>[2x]SQIPASEQET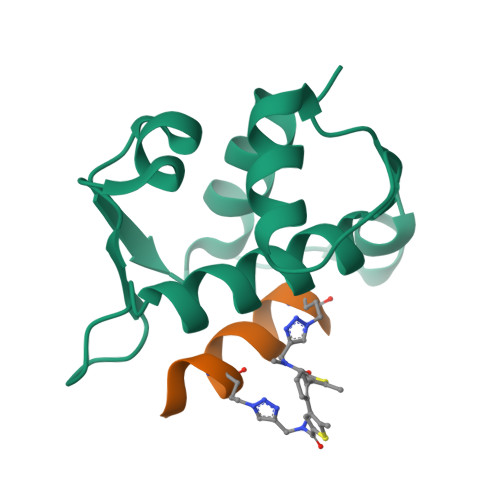LVRPKPLLLKLLKSVGAQKDTYTMKEVLFYLGQYIMTKRLYDAAQQHIVYCSNDLLGDLFGVPSFSVKEHRKIYTMIYRNLV;>XLTFGEYWAQLAS[2x]>MHAFPLTLDNRLAEALPLWRNLARTDRAPRRNIDLADWKADWRELIAALDRFSRSHGYRQPFAAQGHAALENAWAWGQAAENASTLLLKAIDRGLAGAELRSIYLETAALWLDYSRLLGAARDSLREQGEVDFETAPALAPRTGQYPFALQLLAMGVLLDAQELIPALVEEVLQFDTDRLLDYLGAAALGLTSASEETFHPRPFGQLRAFFEEADGSDAQALAPYLQSQYREFFQLSPKAQKKTRRLTGPYAWGWWAMEVSALGVLYGWDDGVL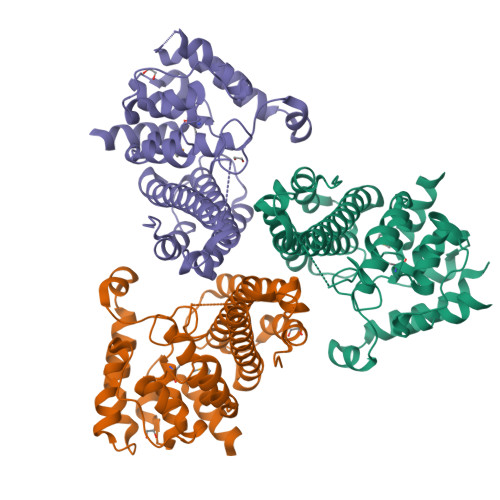RASPHYLGDLVDYARARGDA[3x]5-(2-fluorophenyl)-1,3-oxazole-4-carboxylic acid 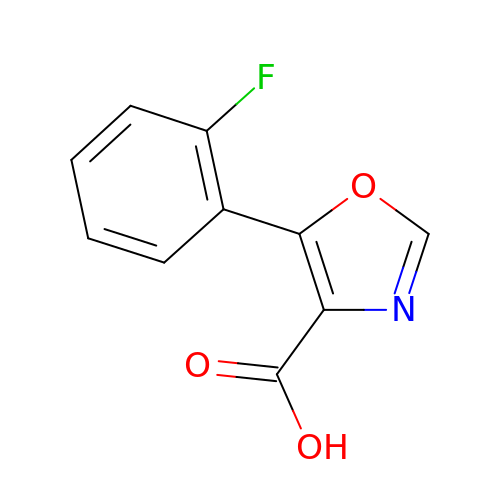| C10 H6 F N O3 | COYYCXFHTJQGGF-UHFFFAOYSA-N>[4x]ADKLPNIVILATGGTIAGSAATGTQTTGYKAGALGVDTLINAVPEVKKLANVKGEQFSNMASENMTGDVVLKLSQRVNELLARDDVDGVVITHGTDTVEESAYFLHLTVKSDKPVVFVAAMRPATAISADGPMNLLEAVRVAGDKQSRGRGVMVVINDRIGSARYITKTNASTLDTFRANEEGYLGVIIGNRIYYQNRIDKLHTTRSVFDVRGLTSLPKVDILYGYQDDPEYLYDA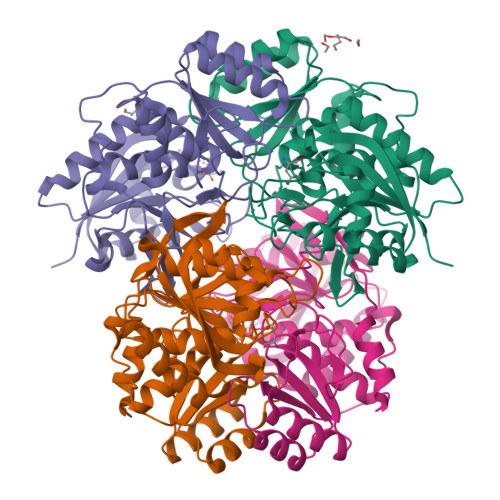AIQHGVKGIVYAGMGAGSVSVRGIAGMRKALEKGVVVMRSTRTGNGIVPPDEELPGLVSDSLNPAHARILLMLALTRTSDPKVIQEYFHTY>KPLQNWEQASPGENAHSSLGLSGAGEEGVFDLQMFLENMKVDFLRSLNLSGIPSQDKTRAEPPQYMIDLYNRYTTDKSSTPASNIVRSFSVEDAISTAATEDFPFQKHILIFNISIPRHEQITRAELRLYVSCQNDVDSTHGLEGSMVVYDVLEDSETWDQATGTKTFLVSQDIRDEGWETLEVSSAVKRWVRADSTTNKNKLEVTVQSHRESCDTLDISVPPGSKNLPFFVVFSNDRSNGTKETRLELKEMIGHEQETMLVKTAKNAYQVAGESQEEEGLDGYTAVGPL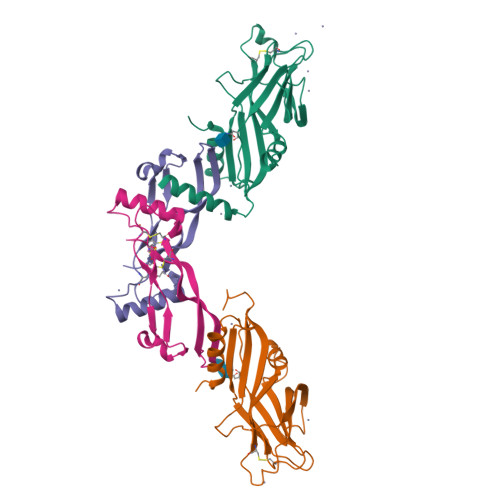LARRKR[2x];>[2x]SAGAGSHCQKTSLRVNFEDIGWDSWIIAPKEYEAYECKGGCFFPLADDVTPTKHAIVQTLVHLKFPTKVGKACCVPTKLSPISVLYKDDMGVPTLKYHYEGMSVAECGCR>[4x]MDLSQLTPRRPYLLRAFYEWLLDNQLTPHLVVDVTLPGVQVPMEYARDGQIVLNIAPRAVGNLELANDEVRFNARFGGIPRQVS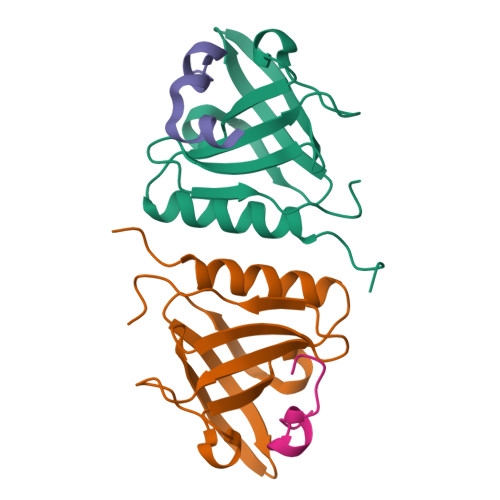VPLAAVLAIYARENGAGTMFEPEAAYDEDTSIMN;>EAQPAPHQWQKMPFWQKVRPWAAQLTQMGVAA[4x]>KETAAAKFERQHMDSSTSPASSSNYCNLMMCCRNLTKDRCKPVNTFVHESLADVQAVCSQKNVACKNGQTNCYQSYSTMSITDCRETGSSKYPNCAYKTTQANKHIIVACEGNPYVPVHFDASV[2x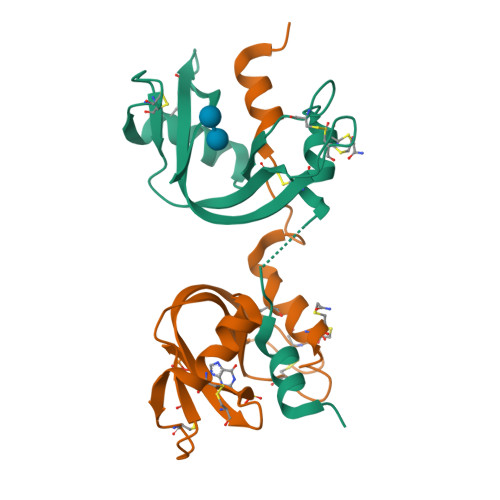]> GSHMWDT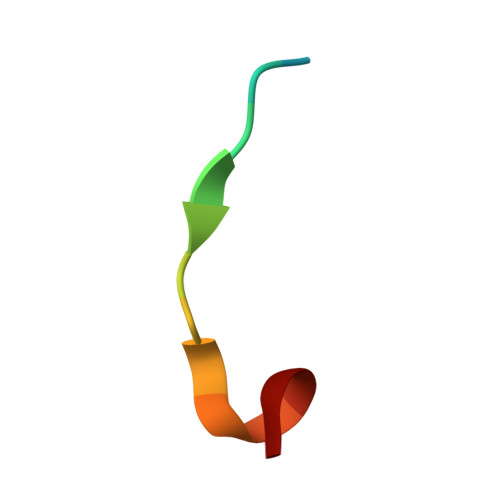ANNPLYKE>[7x]MAPGREEILEMHGLRRIIFDKMTKAKQIMPHFTVMEEVDVTSMVSILDSAKARNRKVTVTGFLARIVPSILKQYPYLNAIYDETRRVYILKKYYNIGIA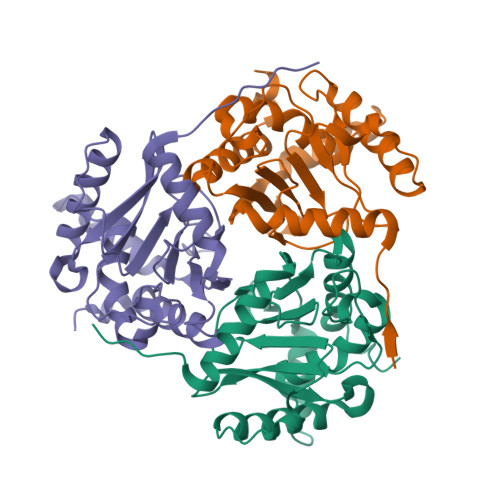VDTPDGLNVFVIKDADRKSMVEISAEISDKASRARENKLQLDEVQDSTFTITNVGTIGGIMSTPIINYPEVAILGVHRILEREGRKYMYLSLSCDHRLIDGAVATRFIVDLKKVIEDPNAIIYEI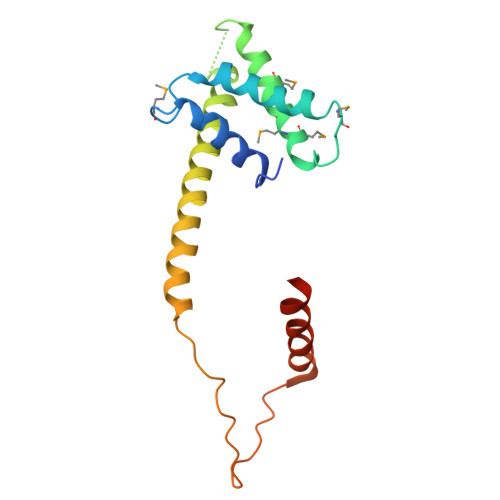> MDIKLKDFEGPLDLLLHLVSKYQMDIYDVPITEVIEQYLAYVSTLQAMRLEVTGEYMVMASQLMLIKSRKLLPKVAEVTDLGDDLEQDLLSQIEEYRKFKLLGEHLEAKHQERAQYYSKAPTELIYEDAELVHDKTTIDLFLAFSNILAKKKEEFAQNHT>SDFANLSSTNKELSPQYNWVACGILEGGLKAAGVLEEGQYNRELAEAIAAKGEGFWTTQFPQIGDWNEDQAAALADRAQT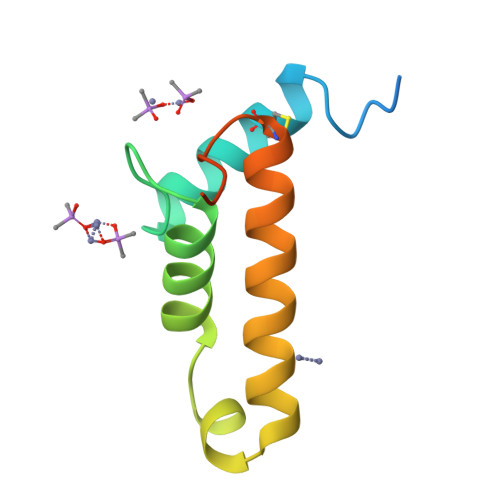CGLVKADTYLSELSSNFSS[9x]> GMQEHYQPAAIEPAAQKKWDDARISNVSEDASKPKYYCLSMFPYPSGKLHMGHVRNYTIGDVLSRFKLLNGFNVMQPMGWDAFGMPAENAAMKNNVAPAAWTYDNIEYMKTQLKSLGFAVDWEREVATCKPEYYRWEQWLFTKLFEKGIVYRKNGTVNWDPVDQTVLANEQVIDGRGWRSGALIEKREIPMYYFKITDYAEELLNDLDKLEHWPEQVKTMQRNWIGKSRGMTVRFAVSDDSKQGLEGDYAKFLQVYTTRPDTLMGATYVAVAAEHPLATAAAADKPELQAFIAECKAGSVAEADMATMEKKGVPTGRYVVNPLNGDKLEVWIANYVLWGYGDGAVMAVPAHDERDFEFAAKYNLPKKQVIAVGDNAFDANRWQEWYGDKENGVLVNSGDLDGLDFQTAFDAVAAKLQSQGAGEPKTQYRLRDWGISRQRYWGCPIPIVHCEKCGNVPVPADQLPVVLPENVVPDGMGSPLAKMPEFYETSCPCCGGAAKRETDTMDTFIESSWYFFRYMSPKFSDGMVSAESAKYWGAVDQYIGGIEHAIAHLLYARFFTKLMRDEGLVNVDEPFERLLTQGMVVCETYYRENDKGGKDWINPADVELTFDDKGRPVSAVLKADGLPVVISGTEKMSKSKNNGVDPQELINAYGADTARLFMMFAAPPEQSLEWSDSGVEGAHRFLRRLWRTVYEYLKQGGAVKAFAGNQDGLSKELKDLRHKLHSTTAKVSDDYGRRQQFNTAIAAVMELLNQYDKTDTGSEQGRAVAQEVLEAAVRLLWPIVPHICETLWSELNGAKLWEAGWPTVDEAALVKSEIEVMVQVNGKLRGKITVAADASKADLEAAALANEGAVKFMEGKPAKKIIVVPGRLVNIVV

To correctly aminoacylate tRNALeu, leucyl-tRNA synthetase (LeuRS) catalyzes three reactions: activation of leucine by ATP to form leucyl-adenylate (Leu-AMP), transfer of this amino acid to tRNALeu and post-transfer editing of any mischarged product. Mechanistically similar to other adenylate-forming enzymes, the class Ia aminoacyl-tRNA synthetase (aaRS) LeuRS charges tRNALeu isoacceptors, which are essential substrates for protein translation. We have solved crystal structures for all enzymatic states of Neisseria gonorrhoeae LeuRS during Leu-AMP formation.

To understand the role of this peptide-plane flip on the global conformational changes and its effects on enzymatic catalysis, L550 was mutated to an alanine or glycine and the crystallization of both mutants was performed. Comparison of the captured apo and pre-transition states of both mutants show the same large domain movement, including closure of the active site by the CP1 hairpin and structurally associated α-helix (M84-N93), that were seen for the WT structures. Despite the occurrence of these substrate-induced changes, including the shift of the priming loop, no peptide-plane flip was observed in either mutant pre-transition state structure. This is likely the result of the absence of the clash between the side chains of E169 of the CP1 hairpin and A550/G550 although the side chain of E169 maintains the same interactions as seen for the WT pre-transition structure. Our biochemical data show that in the absence of steric constraints the peptide-plane flip is not necessary for the amino acid activation.>[4x]SMRPQPGDGERRYREASARKKIRLDRKYIVSCKQTEVPLSVPWDPSNQVYLSYNNVSSLKMLVAKDNWVLSSEISQVRL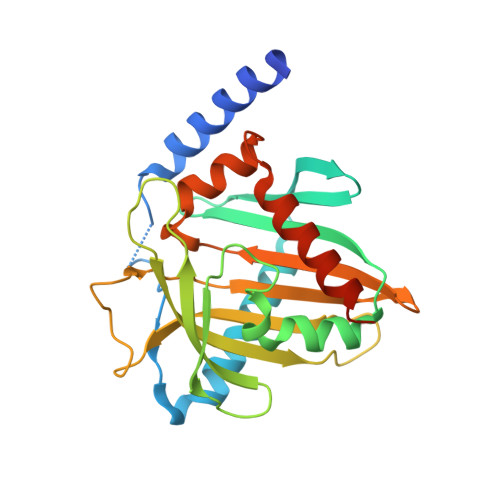YTLEDDKFLSFHMEMVVHVDAAQAFLLLSDLRQRPEWDKHYRSVELVQQVDEDDAIYHVTSPALGGHTKPQDFVILASRRKPCDNGDPYVIALRSVTLPTHRETPEYRRGETLCSGFCLWREGDQLTKVSYYNQATPGVLNYVTTNVAGLSSEFYTTFKACEQFLLDNRNDLAPSLQTL> CGPKRDPYAKAGKSEGKPDKLVVWENADDGVQLNNTKKWAGEFTKKTGIQVEVVPVALLKQQEKLTLDGPAGKGADLVTWPHDRLGEAVTKGLLQPIQVDNSVKNQFDDVAMKALTYGGKLYGLPKAIESVALIYNKKLMGQVPATYDELFQYAKANNKPDEQKYGVLFEANNFYYTYFLFAAKGAAVFKEQDGTLDPNEIGLNSPEAVQGMNEVQKWFTEARLPQSLKADTVNGLFKSGKVAAVINGPWAIKDYQAAGINVGVAPLPKIDGKDA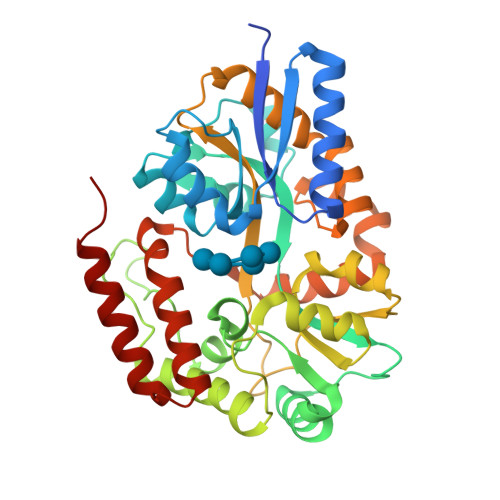QTFIGVKGWYLSAYSKYPKYATELMQFLTSKEALASRFKETGEIPPQKELLNDPMIKNNPVVNGFAKQASKGVPMPSIPEMGVVWEPINNAHTFVAQGKQTPEQALNDAVKIMKEKIQTMKQ(3S)-1-(4-acetylphenyl)-5-oxopyrrolidine-3-carboxylic acid | C13 H13 N O4 | 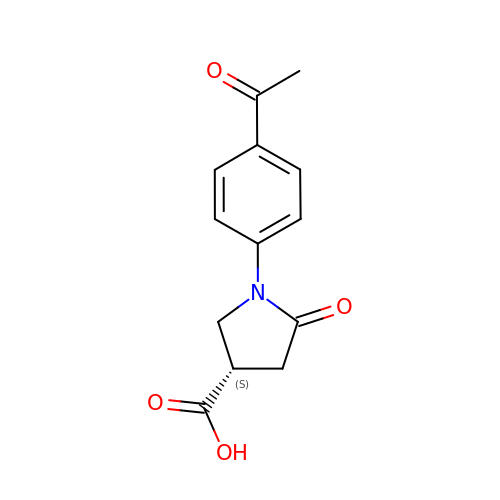SQGYWRZISBCKMW-JTQLQIEISA-N> MCIEFAFKKAGIPIVRNFLHSTEGVIYGLPQRVQRNLAINYTVKQYKEGKAVS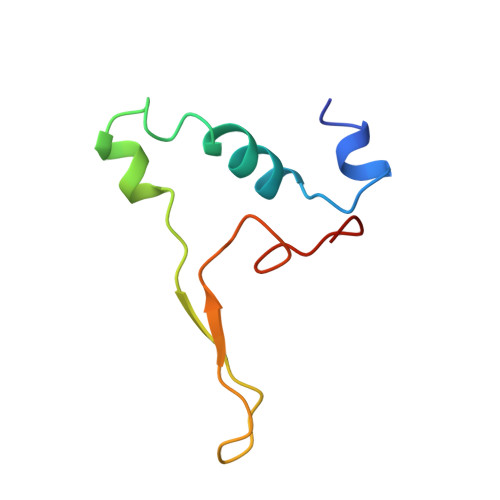AKTIKTLQEAFPSKGDTK> SDTKTSKTVGGRKIINSEFAGKTVTTKGGDVRFDSDGFPDFTPYSKKTVRVIGLTGDMANDVPLAMARA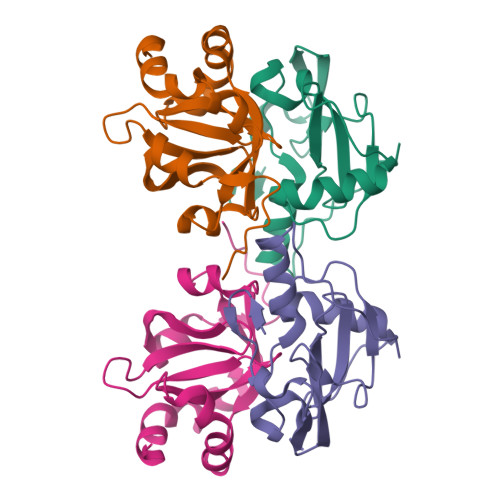KITKYDKSKYVWHHHQDGKTMMLIPKSVHSVRNGGVAHTGGRSVIQHNLLNPNNKLNYSSPEELV;> MISLSDIENLIQHIWEEPIFSDVTSKKVVVSLYGTLSKKIPDKFIIIEEVFPKDELEDIWSNYEEYLDEYLIFPFLGTLGEAVICIGYGNDNKGKIFYFDFDFGACELDGDNLEAFLEKLLESGSTENLYFQ>[2x]MTGGMKPPARKPRILNSDGSSNITRLGLEKRGWLDDHYHDLLTVSRPVFITLITGLYLVTNALFALAYLACGDVIENARPGSFTDAFFFSVQTMATIGYGKLIPIGPLANTLVTLEA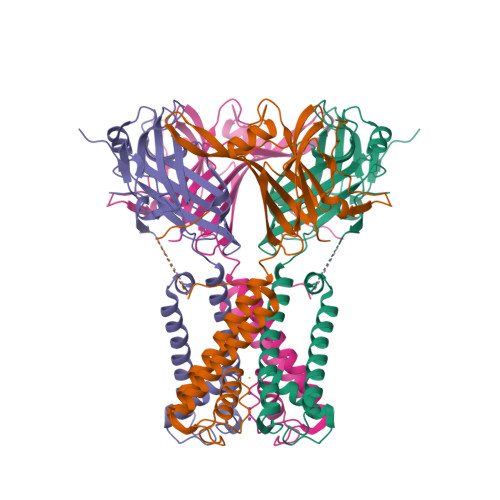LCGMLGLAVAASLIYARFTRPTAGVLFSSRMVISDFEGKPTLMMRLANLRIEQIIEADVHLVLVRSEISQEGMVFRRFHDLTLTRSRSPIFSLSWTVMHPIDHHSPIYGETDETLRNSHSEFLVLFTGHHEAFAQNVHARHAYSCDEIIWGGHFVDVFTTLPDGRRALDLGKFHEIAQHHHHHH> CPEQDKYRTITGMCNNRRSPTLGASNRAFVRWLPAEYEDGFSLPYGWTPGVKRNGFPVALARAVSNEIVRFPTDQLTPDQERSLMFMQWGQLLDHDLDFTPEPAARASFVTGVNCETSCVQQPPCFPLKIPPNDPRIKNQADCIPFFRSCPACPGSNITIRNQINALTSFVDASMVYGSEEPLARNLRNMSNQLGLLAVNQRFQDNGRALLPFDNLHDDPCLLTNRSARIPCFLAGDTRSSEMPELTSMHTLLLREHNRLATELKSLNPRWDGERLYQEARKIVGAMVQIITYRDYLPLVLGPTAMRKYLPTYRSYNDSVDPRIANVFTNAFRYGHTL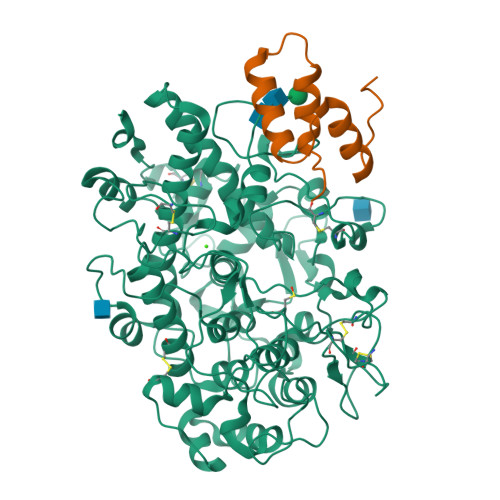IQPFMFRLDNRYQPMEPNPRVPLSRVFFASWRVVLEGGIDPILRGLMATPAKLNRQNQIAVDEIRERLFEQVMRIGLDLPALNMQRSRDHGLPGYNAWRRFCGLPQPETVGQLGTVLRNLKLARKLMEQYGTPNNIDIWMGGVSEPLKRKGRVGPLLACIIGTQFRKLRDGDRFWWENEGVFSMQQRQALAQISLPRIICDNTGITTVSKNNIFMSNSYPRDFVNCSTLPALNLASWRE;> ANFLEHELSYIDVLLDKNADQATKDNLRSYFADKGLHSIKDIINKAKQDGFDVSKYEHVK>[4x]GPGSCPTHADSLNNLANIKREQGNIEEAVRLYRKALEVFPEFAAAHSNLASVLQQQGKLQEALMHYKEAIRISPTFADAYSNMGNTLKEMQDVQGALQCYTRAIQINPAFADAHSNLASIHKDSGNIPEAIASYRTALKLKPDFPDAYCNLAHCLQIVCDWTDYDERMKKLVSIVADQLEKNRLPSVHPHHSMLYPLSHGFRKAIAERHGNLCLDKINVLHKPPYEHPKDLKLSDGRLRVGYVSSDFGNHPTSHLMQSIPGMHNPDKFEVFCYALSPDDGTNFRVKVMAEANHFIDLSQIPCNGKAADRIHQDGIHILVNMNGYTKGARNELFALRPAPIQAMWLGYPGTSGALFMDYIITDQETSPAEVA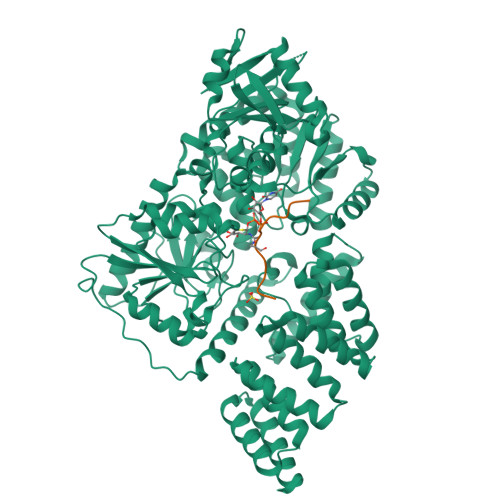EQYSEKLAYMPHTFFIGDHANMFPHLKKKAVIDFKSNGHIYDNRIVLNGIDLKAFLDSLPDVKIVKMKCPDGGDNADSSNTALNMPVIPMNTIAEAVIEMINRGQIQITINGFSISNGLATTQINNKAATGEEVPRTIIVTTRSQYGLPEDAIVYCNFNQLYKIDPSTLQMWANILKRVPNSVLWLLRFPAVGEPNIQQYAQNMGLPQNRIIFSPVAPKEEHVRRGQLADVCLDTPLCNGHTTGMDVLWAGTPMVTMPGETLASRVAASQLTCLGCLELIAKNRQEYEDIAVKLGTDLEYLKKVRGKVWKQRISSPLFNTKQYTMELERLYLQMWEHYAAGNKPDHMIKPVE;>PVSVPYASAQSTS[4x]>RSEAPRRPSRKGLRNDKDKPLPPLLARVGGNIEVLGFNARQRKAFLNAIMRYGMPPQDAFTTQWLVRDLRGKSEKEFKAYVSLFMRHLCEPGADGAETFADGVPREGLSRQHVLTRIGVMSLIRKKVQEFEHVNGRWSMPELAEVEENKKMSQPGSPSPKTPTPSTPGDTQPNTPAPVPPAEDGIKIEENSLKEEESIEGEKEVKSTAPETAIECTQAPAPASEDEKVVVEPPEGEEKVEKAEVKERTEEPMETEPKGAADVEKVEEK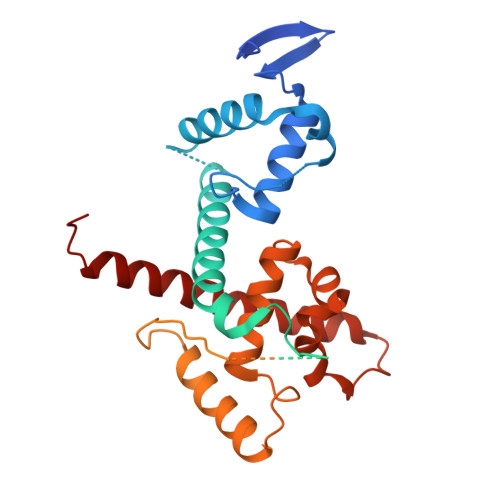SAIDLTPIVVEDKEEKKEEEEKKEVMLQNGETPKDLNDEKQKKNIKQRFMFNIADGGFTELHSLWQNEERAATVTKKTYEIWHRRHDYWLLAGIINHGYARWQDIQNDPRYAILNEPFKGEMNRGNFLEIKNKFLARRFKLLEQALVIEEQLRRAAYLNMSED[2x]> APPNLWAAQ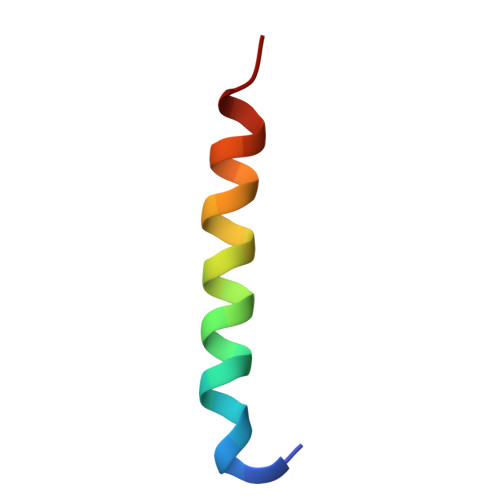RYGRELRRMSDEFEGSFK Siderocalin/Lipocalin 2/Neutrophil Gelatinase Associated Lipocalin/24p3 is an innate immune system protein with bacteriostatic activity, acting by tightly binding and sequestering diverse catecholate and mixed-type ferric siderophores from enteric bacteria and mycobacteria. Despite limited sequence similarity beyond minimal fold-defining motifs, lipocalins, including Scn (Coles et al., 1999, Goetz et al., 2000), display a common structural architecture: an eight-stranded antiparallel β-barrel enclosing a cup-shaped ligand binding site, or calyx. The calyx is strongly electropositive overall, due to the close arrangement of the side-chains of two lysines (K125, K134) and an arginine (R81), which complements the net negative charge of many ferric siderophores. Scn displays exceptional structural rigidity, manifested by its near-identical structure across multiple crystal structures, bound to a series of distinct ligands, tolerating multiple mutations.

The Scn calyx side-chains most closely contacting ligands are K125 and K134, together bracketing Pocket #1, W79 and R81, typically swapping rotamers to divide Pockets #2 and #3, and Y106, creating the central floor of the calyx under the chelated metal. We had previously determined Fe-ENT KDs and co-crystal structures for the Scn(C87S/W79A/R81A) and Scn(C87S/Y106F) mutants. The W79A/R81A mutation reduced the affinity for Fe-ENT ∼175-fold, from 0.4 nM to 71 nM, and the Y106F mutation reduced the affinity ∼50-fold, from 0.4 nM to 20 nM. The structure of the Scn(C87S/W79A/R81A) mutant was quite similar to that of wild-type Scn, with the affinity reduction readily accounted for simply by the loss of W79 and R81 contacts and interactions. The structure of the minimal Scn(C87S/Y106F) mutant, however, was dramatic and surprising, showing complete loss of bound iron and two of three CAM substituents from degraded ENT. This result remains difficult to reconcile, as the only ligand contact involving the hydroxyl of Y106 is a hydrogen bond to the 3-hydroxyl of the CAM substituent in Pocket #1. Overall, this combination mutant showed ligand features similar in essential details to the Scn(C87S/Y106F) mutant. None of these mutations noticeably altered the Scn fold.

>MPLGLLWLGLALLGALHAQAQDSTSDLIPAPPLSKVPLQQNFQDNQFQGKWYVVGLAGNAILREDKDPQKMYATIYELKEDKSYNVTSVLFRKKKCDYAIATFVPGSQPGEFTLGNIKSYPGLTSFLVRVVSTNYNQHAMVFFKKVSQNREYFKITLYGRTKELTSELKENFIRFSKSLGLPENHIVFPVPIDQCIDG[3x]> SSPLPLVVNTWPFKNATEAAWRALASGGSALDAVESGCAMCEREQCDGSVGFGGSPDELGETTLDAMIMDGTTMDVGAVGDLRRIKNAIGVARKV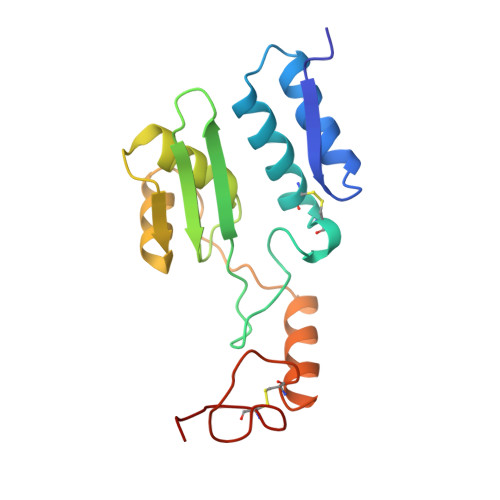LEHTTHTLLVGESATTFAQSMGFINEDLSTSASQALHSDWLARNCQPNYWRNVIPDPSKYCGPYKPP> HHHHHHSSGLVPRGSHMASKIDYLTLFPEMFDGVLNHSIMKRAQENNKLQINTVNFRDYAINKHNQVDDYPYGGGQGMVLKPEPVFNAMEDLDVTEQTRVILMCPQGEPFSHQKAVELSKADHIVFICGHYEGYDERIRTHLVTDEISMGDYVLTGGELPAMTMTDAIVRLIPGVLGNEQSHQDDSFSDGLLEFPQYTRPREFKGLTV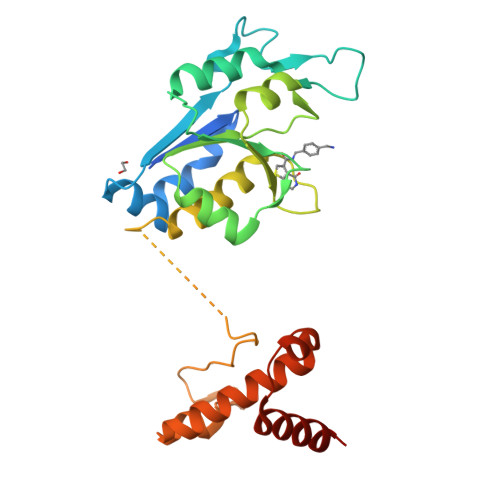PDVLLSGNHANIDAWRHEQKLIRTYNKRPDLIEKYPLTNADKQILERYKIGLKKG>MHHHHHHHDGTENPIHDRTSDYHKYLKVKQGDSDLFKLTVSDKRYIWYNPDPKERDSYECGEIVSETSDSFTFKTVDGQDRQVKKDDANQRNPIKFDGVEDMSELSYLNEPAVFHNLRVRYNQDLIYTYSGLFLVAVNPFKRIPIYTQEMVDIFKGRRRNEVAPHIFAISDVAYRSMLDDRQNQSLLITGESGAGKTENTKKVIQYLASVAGRNQANGSGVLEQQILQANPILEAFGNAKTTRNNNSSRFGKFIEIQFNSAGFISGASIQSYLLEKSRVVFQSETERNYHIFYQLLAGATAEEKKALHLAGPESFNYLNQSGCVDIKGVSDSEEFKITRQAMDIVGFSQEEQMSIFKIIAGILHLGNIKFEKGAGEGAVLKDKTALNAASTVFGVNPSVLEKALMEPRILAGRDLVAQHLNVEKSSSSRDALVKALYGRLFLWLVKKINNVLCQERKAYFIGVLDISGFEIFKVNSFEQLCINYTNEKLQQFFNHHMFKLEQEEYLKEKINWTFIDFGLDSQATIDLIDGRQPPGILALLDEQSVFPNATDNTLITKLHSHFSKKNAKYEEPRFSKTEFGVTHYAGQVMYEIQDWLEKNKDPLQQDLELCFKDSSDNVVTKLFNDPNIASRAKKGANFITVAAQYKEQLASLMATLETTNPHFVRCIIPNNKQLPAKLEDKVVLDQLRCNGVLEGIRITRKGFPNRIIYADFVKRYYLLAPNVPRDAEDSQKATDAVLKHLNIDPEQYRFGITKIFFRAGQLARIEEAREQRLESNEPPMDFDDDIPF[2x]

Myosin is a ubiquitously expressed adenosine triphosphate (ATP)-driven motor protein, producing force and directed motion along cytoskeletal actin filament tracks by converting chemical energy from ATP hydrolysis into mechanical work. Despite their specialized cellular functions, all members of the myosin superfamily share a common multistep mechanism of force generation—the chemomechanical actomyosin motor cycle. The myosin motor is thus subject to substantial conformational changes along that cycle, traversing through different actin-attached and –detached states, eventually amplifying them to a large scale rotation of the converter domain and swinging of the adjacent lever arm in the force-generating power stroke. ADP release is key for the regulation of the mechanical motor function of myosin as it controls the fraction of time the motor stays attached to the actin filament.

The overall conformation highly resembled the previously solved structure of a myosin-II-dynamin fusion construct (root mean square deviation (rmsd) 0.54 (chain A) and 0.57 (chain B)), which was assigned earlier as the Dd myosin-II rigor-like state, with the converter in the down position and the relay helix straightened. A twisted transducer in our crystal structure primed the nucleotide-free active site for binding of ATP, with an intact critical salt-bridge between switch-1 (residue Arg238) and switch-2 (residue Glu459), which has been suggested to play a central role during Pi release. The P-loop (179GESGAKT186) moved away from the switches together with the N-terminal domain. In our rigor-like apo myosin-II structure, the interactions of Arg232 differ markedly from the blebbistatin-bound myosin-II·ADP structure. While Arg232 in the rigor-like state is hydrogen-bonded to Asn674 of the SH2-helix as well, the contact with Glu180 (P-loop) is broken. Instead, Arg232 formed a hydrogen bond with the backbone of Ile460 (switch-2), while Glu180 of switch-1 interacts with Gly457 (switch-2). Hence, both interactions in the rigor-like state assist the maintenance of the closed conformation of the switches, highlighting the central role of the interaction network mediated by Arg232 in chemomechanical coupling in myosin.>[3x]MLKIISANVNGIRSAYKKGFYEYIAASGADIVCVQELKAQEADLSADMKNPHGMHGHWHCAEKRGYSGVAVYSKRKPDNVQIGMGIEEFDREGRFVRCDFGRLSVISLYLPSGSSAEERQQVKYRFLDAFYPMLEAMKNEGRDIVVCGDWNIAHQNIDLKNWKGNQKNSGFLPEEREWIG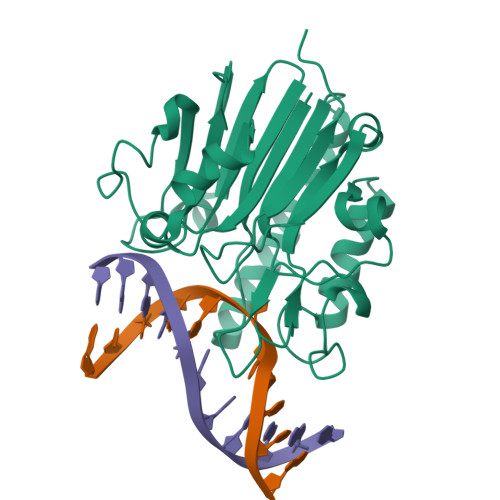KVIHKLGWTDMWRTLYPDVPGYTWWSNRGQAYAKDVGWRIDYQMVTPELAAKAVSAHVYKDEKFSDHAPLVVEYDYAAE> MKPKRVQGKIVIE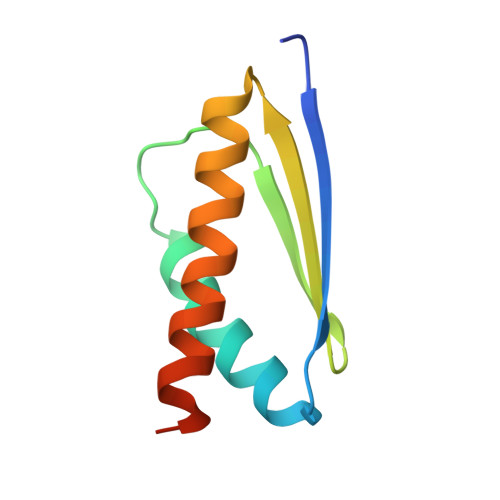FPSEDIAEVVYTSVLYEHVSVPYRRSRVNFRREGRRIVLEIEANDSSAMRGTVNSYLRWIKVALDVLNIHHHHHH{2-[(phosphonomethyl)carbamoyl]-1H-benzo[g]indol-1-yl}acetic acid | C16 H15 N2 O6 P | 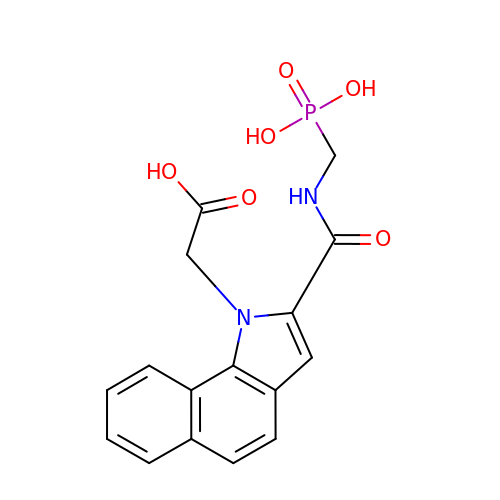JUZJWGPHICAWME-UHFFFAOYSA-N>MVKLAEFSRTATFAWSHDKIPLLVSGTVSGTVDANFSTDSSLELWSLLAADSEKPIASLQVDSKFNDLDWSHNNKIIAGALDNGSLELYSTNEANNAINSMARFSNHSSSVKTVKFNAKQDNVLASGGNNGEIFIWDMNKCTESPSNYTPLTPGQSMSSVDEVISLAWNQSLAHVFASAGSSNFASIWDLKAKKEVIHLSYTSPNSGIKQQLSVVEWHPKNSTRVATATGSDNDPSILIWDLRNANTPLQTLNQGHQKGILSLDWCHQDEHLLLSSGRDNTVLLWNPESAEQLSQFPARGNWCFKTKFAPEAPDLFACASFDNKIEVQTLQNLTNTLDEQETETKQQESETDFWNNVSREESKEKPTVFHLQAPTWYGEPSPAAHWAFGGKLVQITPDGKGVSITNPKISGLESNTTLSEALKTKDFKPLINQRLVKVIDDVNEEDWNLLEKLSMDGTEEFLKEALAFDNDESDAQDDANNEKEDDGEEFFQQIETNFQPEGDFSLSGNIEQTISKNLVSGNIKSAVKNSLENDLLMEAMVIALDSNNERLKESVKNAYFAKYGSKSSLSRILYSISKREVDDLVENLDVSQWKFISKAIQNLYPNDIAQRNEMLIKLGDRLKENGHRQDSLTLYLAAGSLDKVASIWLSEFPDLEDKLKKDNKTIYEAHSECLTEFIERFTVFSNFINGSSTINNEQLIAKFLEFINLTTSTGNFELATEFLNSLPSDNEEVKTEKARVLIASGKSLPAQNPATATTSKAKYTNAKTNKNVPVLPTPGMPSTTSIPSMQAPFYGMTPGASANALPPKPYVPATTTSAPVHTEGKYAPPSQPSMASPFVNKTNSSTRLNSFAPPPNPYATATVPATNVSTTSIPQNTFAPIQPGMPIMGDYNAQSSSIPSQPPINAVSGQTPHLNRKANDGWNDLPLKVKEKPSRAKAVSVAPPNILSTPTPLNGIPANAASTMPPPPLSRAPSSVSMVSPPPLHKNSRVPSLVATSESPRASISNPYAPPQSSQQFPIGTISTANQTSNTAQVASSNPYAPPPQQRVATPLSGGVPPAPLPKASNPYAPTATTQPNGSSYPPTGPYTNNHTMTSPPPVFNKPPTGPPPISMKKRSNKLASIEQNPSQGATYPPTLSSSASPLQPSQPPTLASQVNTSAENVSHEIPADQQPIVDFLKEELARVTPLTPKEYSKQLKDCDKRLKILFYHLEKQDLLTQPTIDCLHDLVALMKEKKYKEAMVIHANIATNHAQEGGNWLTGVKRLIGIAEATLN[2x];>[2x]MVVIANAHNELIHDAVLDYYGKRLATCSSDKTIKIFEVEGETHKLIDTLTGHEGPVWRVDWAHPKFGTILASCSYDGKVLIWKEENGRWSQIAVHAVHSASVNSVQWAPHEYGPLLLVASSDGKVSVVEFKENGTTSPIIIDAHAIGVNSASWAPATIEEDGEHNGTKESRKFVTGGADNLVKIWKYNSDAQTYVLESTLEGHSDWVRDVAWSPTVLLRSYLASVSQDRTCIIWTQDNEQGPWKKTLLKEEKFPDVLWRASWSLSGNVLALSGGDNKVTLWKENLEGKWEPAGEVHQ

COPII mediates Endoplasmic Reticulum to Golgi trafficking of thousands of cargoes. ER export is mediated by the coat protein complex II (COPII), which minimally comprises five cytosolic proteins that form two concentric layers on the ER membrane—the inner and outer coat. The inner coat layer consists of the small GTPase Sar1 and the heterodimeric Sec23/24 complex, whilst the outer coat layer comprises the rod-shaped heterotetramer Sec13/31. Here we visualise the complete, membrane-assembled COPII coat by cryo-electron tomography and subtomogram averaging, revealing the full network of interactions within and between coat layers.

We therefore analysed the structure of the interconnecting rods by focusing the refinements at the mid-points between vertices. At this resolution we can distinguish helical profiles and individual blades of the Sec13 β-propeller. Surprisingly, we detected a previously unresolved extra density attached to the rod halfway between Sec13 and the dimerisation interface. The size of this appendage is indicative of a full domain. The average of Sec31-ΔCTD rods recovers the characteristic features and has similar resolution to the wild-type rod, but it lacks the appendage density (orange arrowhead), confirming this density most likely corresponds to the CTD. Since no atomic model for the Sec31 CTD has been determined, we built a homology model to fit into the appendage density. Rigid-body fitting the homology model in the appendage density shows consistency of size and features, although at this resolution we cannot determine the precise molecular interface. We show that Sec31 CTD is as an essential node of the outer coat network that binds to Sec31 α-solenoid domains. When the truncated form was the sole copy of Sec31 in yeast, cells were not viable, indicating that the interaction we detect is essential for COPII coat function. In contrast, when the cargo burden was decreased by deletion of the ER export receptor, Emp24, Sec31-ΔCTD supported viability. This phenotype is similar to the depletion of the Sec31-ΔNTD or of Sec1326, and leads us to hypothesise that Sec31 CTD binding to Sec31 rods stabilises the COPII interaction network, thereby imparting rigidity and strengthening the coat.> SCPPTKFQCRTSGLCVPLTWRCDRDLDCSDGSDEEECRIEPCTQKGQCPPPPGLPCPC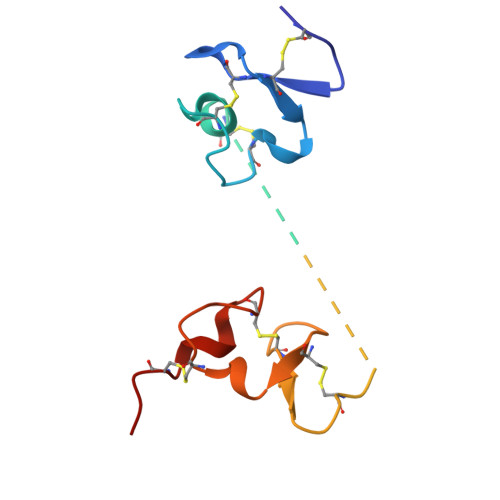TGVSDCSGGTDKKLRNCSRLACLAGELRCTLSDDCIPLTWRCDGHPDCPDSSDELGCGTNE>[4x]SNDIYFNFQRFNETNLILQRDASVSSSGQLRLTNLNGNGEP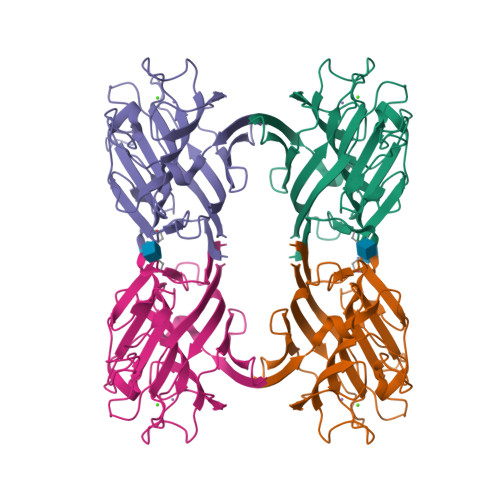RVGSLGRAFYSAPIQIWDNTTGTVASFATSFTFNIQVPNNAGPADGLAFALVPVGSQPKDKGGFLGLFDGSNSNFHTVAVEFDTLYNKDWDPTERHIGIDVNSIRSIKTTRWDFVNGENAEVLITYDSSTNLLVASLVYPSQKTSFIVSDTVDLKSVLPEWVSVGFSATTGINKGNVETNDVLSWSFASKLS>MISNSSAESISAPPNDSTIPHLAIDPFSLDFFDDPYPDQQTLRDAGPVVYLDKWNVYGVARYAEVHAVLNDPTTFCSSRGVGLSDFKKEKPWRPPSLILEADPPAHTRPRAVLSKVLSPATMKTIRDGFAAAADAKVDELLQRGCIDAIADLAEAYPLSVFPDAMGLKQEGREHLLPYAGLVFNAFGPPNELRQTAIERSAPHQAYVNEQCQRPNLAPGGFGACIHAFTDTGEITPDEAPLLVRSLLSAGLDTTVNGIGAAVYCLARFPGELQRLRSDPTLARNAFEEAVRFESPVQTFFRTTTREVELGGAVIGEGEKVLMFLGSANRDPRRWSDPDLYDITRKTSGHVGFGSGVHMCVGQLVARLEGEVMLSALARKVAAIDIDGPVKR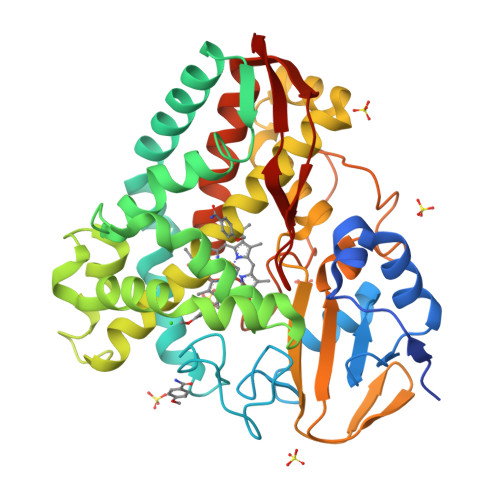RFNNTLRGLESLPVKLTPA[4x]> CAAATVRIAGRDGFCA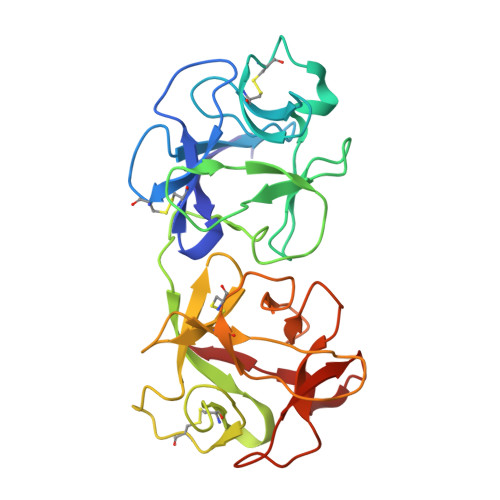DVNGEGQNGAAIILKKCAENDNQLWTLKREATIRSNGGCLTTAAAEQAKAGIYDCTQATAELSAWEIADNGTIINPASSLVLSSGAANSLLDLGVQTNSYASAQGWRTGNETSASVTQISGSAQLCMQAGNGPANLWMSECRAGKAEQQWALLTDKSIRSETNSDNCLTSAADAGPKTILLALCSGPASQRWVFDDDGSILSLYDDKQMDSEGAAAAAKQIILWWNAAEPNQIWLALF> MIIKGRAHKFGDDVDTDAIIPGPYLRTTDPYELASHCMAGIDENFPKKVKEGDVIVAGENFGCGSSREQAVIAIKYCGIKAVIAKSFARIFYRNAINVGLIPIIANTDEIKDGDIVEIDLDKEEIVITNKNKTIKCETPKGLEREILAA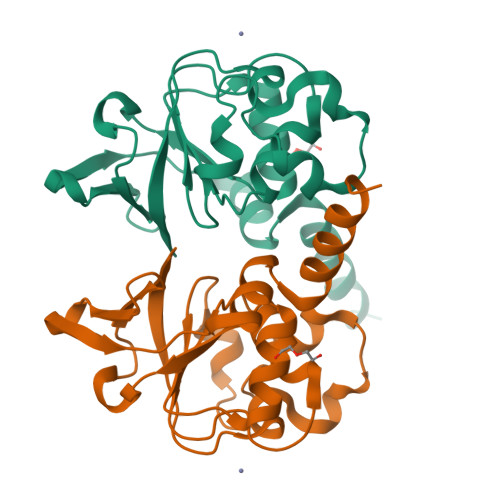GGLVNYLKKRKLIQSKKGVKT>[4x]GGSMLTLIQGKKIVNHLRSRLAFEYNGQLIKILSKNIVAVGSLRREEKMLNDVNLLIIVPEKKLLKHVLPNIRIKGLSFSVKVCGE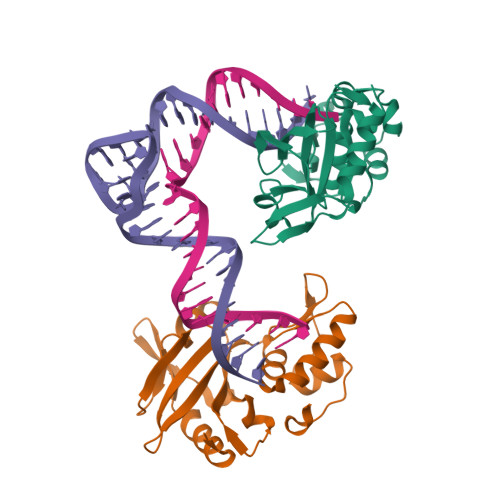RKCVLFIEWEKKTYQLDLFTALAEEKPYAIFHFTGPVSYLIRIRAALKKKNYKLNQYGLFKNQTLVPLKITTEKELIKELGFTYRIPKKRL> MGHHHHHHMALERSDVEKIAHLAR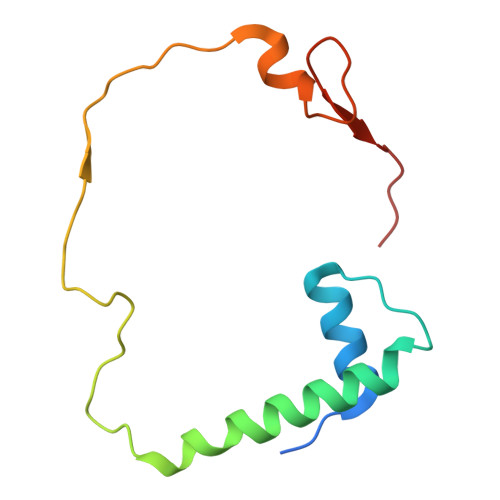LGLSEADLPRTTETLNNILGLIDQMQAVDTSGVEPLAHPLEATQRLRPDAVTETDHRDAYQTIAPAVEEGLYLVPKVIES>MYTNSDFVVIKALEDGVNVIGLTRGADTRFHHSEKLDKGEVLIAQFTEHTSAIKVRGKAYIQTRHGVIESEGKKAAAAAAA[6x];>[9x]MVIATDDLEVACPKCERAGEIEGTPC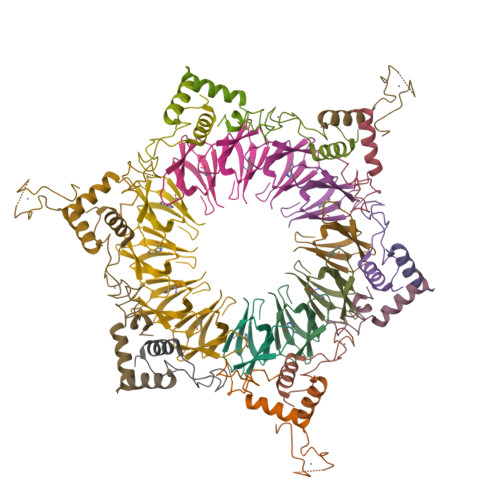PACSGKGVILTAQGYTLLDFIQKHLNK QUINOLINIC ACID | 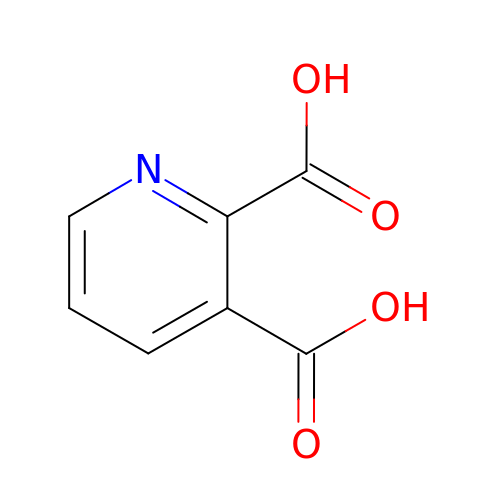C7 H5 N O4 | GJAWHXHKYYXBSV-UHFFFAOYSA-N> GAAGGAGDKLHATPGMFVQHSTAIFSDRYKGQRVLGKGSFGEVILCKDKITGQECAVKVISKRQVKQKTDKESLLREVQLLKQLDHPNIMKLYEFFEDKGYYYLVGEVYTGGELFDEIISRKRFSEVDAARIIRQVLSGITYMHKNKIVHRDLKPENLLLESKSKDANIRIIDFGLSTHFEASKKMKDKIGTAYYIAPEVLHGTYDEKCDVWSTGVILYILLSGCPPFNGANEYDILKKVEKGKYTFELPQWKKVSESAKDLIRKMLTYVPSMRISARDALDHEWIQTYTKEQISVDVPSLDNAILNIRQFQGTQKLAQAALLYMGSKLTSQDETKELTAIFHKMDKNGDGQLDRAELIEGYKELMKMKGQDASML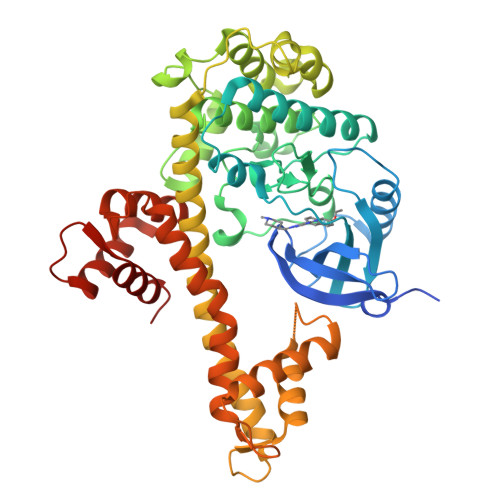DASAVEHEVDQVLDAVDFDKNGYIEYSEFVTVAMDRKTLLSRERLERAFRMFDSDNSGKISSSELATIFGVSDVDSETWKNVLAEVDKNNDGEVDFDEFQQMLLKLCGN1'-((1,4-DIDEOXY-1,4-IMINO-D-ARABINITOL)-4-N-AMMONIUM)-1'-DEOXY-L-ERYTHRITOL-3'-SULFATE INNER SALT | C9 H18 N O9 S | 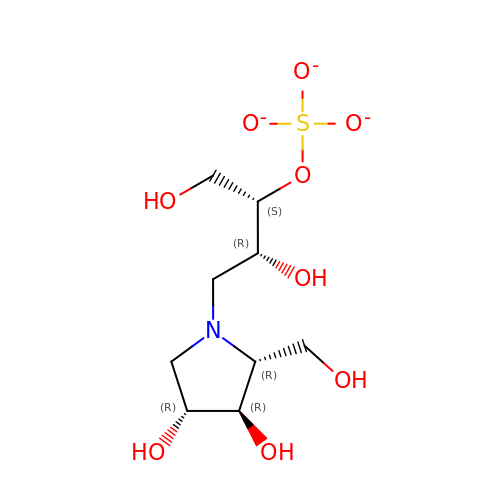YWOSRVQDYDWMAB-JBXPSPKUSA-K>MHHHHHHGPLPDAKPLVEEATAQTKALKSAHMVLTVNGKIPGLSLKTLSGDLTTNPTAATGNVKLTLGGSDIDADFVVFDGILYATLTPNQWSDFGPAADIYDPAQVLNPDTGLANVLANFADAKAEGRDTINGQNTIRISGKVSAQAVNQIAPPFNATQPV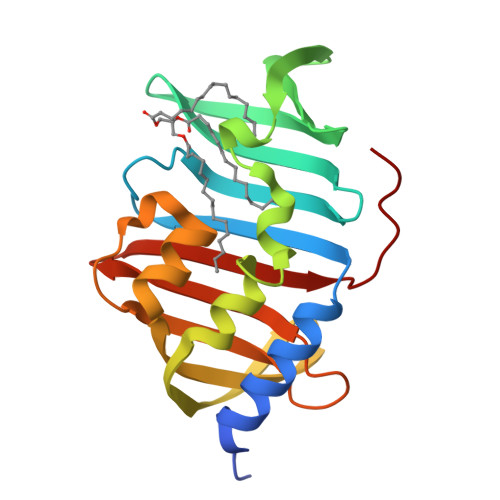PATVWIQETGDHQLAQAQLDRGSGNSVQMTLSKWGEKVQVT[2x]4-methyl-6-(2-(5-(1-methylpiperidin-4-yl)pyridin-3-yl)ethyl)pyridin-2-amine | C19 H26 N4 | 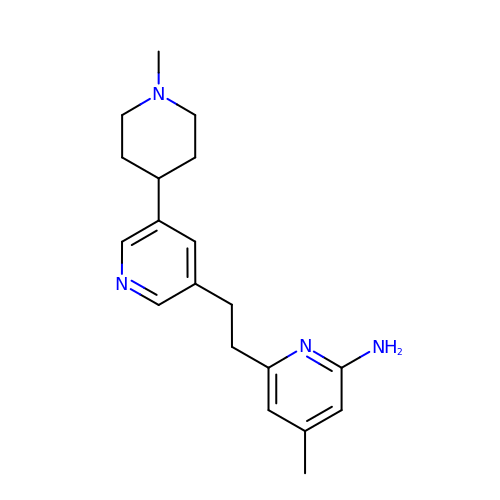UTFTUBTWHNJKBO-UHFFFAOYSA-N> GGCGAAGAAC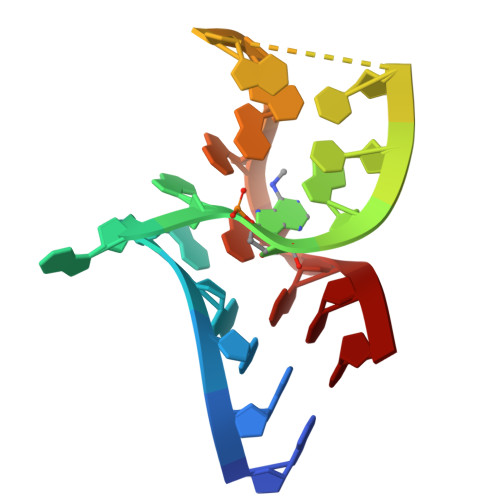CGGGGAGCC>[2x]ATPLTSLGSEQAMFHGKHQPGITTPMQARGHLVAFDLAAGAGRKEAAALLRRWSDTARRLMAGEPAGSRDTDVARDAGPSSLTVTFGFGHSFFGRTGLEKQRPVALDPLPDFSSDHLDKNRSNGDLWVQIGADDALVAFHALRAIQRDAGAAARVRWQMNGFNRSPGATAHPMTARNLMGQVDGTRNPKPGEADFDRRIFVPEEPEAGKGGPAWMANGSYVVVRRIRMLLDDWEELSLKAQEDVIGRRKSDGAPLSGGSGATESTEMDLEKTDGSGELVVPINAHARITRPDQNGGAAMVRRPFSYHDGFDADGVPDAGLLFVCWQADPLRGFVPVQRKLDRGDALSQFIRHEASGLFAVPGGAAEGEYVGQRLLEG

Furthermore, in situ X-ray-driven generation of haem intermediates in crystals of the dye-decolourizing-type peroxidase A (DtpA) from Streptomyces lividans is described. We describe the use of online UV–visible spectroscopy to monitor the X-ray-generated formation of an oxyferrous complex of the dye-decolorizing-type peroxidase A (DtpA) from Streptomyces lividans, allowing its structural characterization. High-resolution crystal structures determined using synchrotron radiation are central to our understanding of haem-protein function. The correct assignment of crystal structures to the correct protein redox and ligand states is essential to avoid the misinterpretation of structural data. This is a particular concern for haem proteins, which can occupy a wide range of redox states and are exquisitely sensitive to becoming reduced by solvated electrons generated from interactions of X-rays with water molecules in the crystal.

Therefore, the observation of this band together with the λmax of the Soret band are strong support for the crystal being in the ferric haem oxidation state. For the present crystal the 0.99 MGy initial structure has two molecules in the crystallo­graphic asymmetric unit, denoted here as A and B, and has been determined to 1.45 Å resolution. An electron-density feature at the distal haem face already suggests the formation of a six-coordinate species, with some extra electron density assigned to a partially populated H2O molecule. Examination of the electron-density maps and structures for the two successive DtpA structures (with accumulated doses of 0.99 and 1.98 MGy, respectively) revealed no substantial differences in coordinates or B factors and no appreciable signs of specific radiation damage beyond the haem pocket. For crystals of DtpA, clear differences were apparent in the spectra of different haem states between room-temperature solution and 100 K structures. The structures allowed the assignment of 100 K spectra to either a diatomic (oxygen) or monatomic (compound III) state, while the spectra allowed X-ray and ligand-soaking effects to be precisely monitored.> GSNNVLPTWSLDSNGEMRSRLSLSEVLDSGDLMKFAVDKTGCQFLEKAVKGSLTSYQKFQLFEQVIGRKDDFLKLSTNIFGNYLVQSVIGISLATNDDGYTKRQEKLKNFISSQMTDMCLDKFACRVIQSSLQNMDLSLACKLVQALPRDARLIAICVDQNANHVIQKVVAVIPLKNWEFIVDFVATPEHLRQICSDKYGCRVVQTIIEKLTADSMNVDLTSAAQNLRERALQRLMTSVTNRCQELATNEYANYIIQHIVSNDDLAVYRECIIEKCLMRNLLSLSQEKFASHVVEKAFLHAPLELLAEMMDEIFDGYIPHPDTGKDALDIMMFHQFGNYVVQCMLTICCDAVSGRRQTKEGGYDHAISFQDWLKKLHSRVTKERHRLSRFSSGKKMIETLANLRSTHPIYELQSSGHDSFKTDYFSTASEHDGPELEKNGIEEGSLMLEPRSNKSSVSVKFSSSGSHGDD

Caenorhabditis elegans PUF protein fem-3 binding factor-2 (FBF-2) partners with intrinsically disordered Lateral Signaling Target-1 (LST-1) to regulate target mRNAs in germline stem cells. FBF-2 has an architecture characteristic of all PUF proteins, including Drosophila Pumilio and human PUM1 and PUM2. The signature PUF RNA-binding domain (RBD), also called the Pumilio-Homology Domain (PUM-HD), is flanked by extended N-terminal and short C-terminal IDRs. The PUF RBD with eight α-helical repeats recognizes RNA sequence elements.

To explore possible roles of the FBF-2 CT, we expressed and purified an FBF-2 fragment containing both RBD and CT (FBF-2164–632). We determined a crystal structure of FBF-2 RBD + CT in complex with a cFBE RNA (5′-CUGUGAAUG-3′) at 2.1 Å resolution. The electron density map revealed new density, not present in the previous RBD structures. This additional density appeared near a loop in the RBD that connects repeats 7 and 8. The sequence of FBF-2 CT residues 607-613 matched this new electron density, but other C-terminal residues (aa 570-606 and 614-632) were disordered. In the FBF-2 RBD + CT/cFBE crystal structure, the seven visible FBF-2 CT residues (SLMLEPR607–613) align structurally with the core regions of LST-1 A (residues 32-38) and LST-1 B (residues 80-86) and made remarkably similar contacts to the RBD. FBF-2 L610 occupied the same position as the key leucines, L35 and L83, in the LST-1 A and B PIMs, and like LST-1 A L35 and LST-1 B L83, FBF-2 L610 was seated in a hydrophobic binding pocket formed by the Y479, L444, I492, and H482 residues of FBF-2. FBF-2 RBD residues Q448, G478, and I480 contacted the peptide backbone atoms of the FBF-2 CT, LST-1 A, and LST-1 B. Thus, the FBF-2 CT contains an intrinsic PIM. We propose that the FBF-2 PIM acts as Velcro®, attaching to the RBD and constraining the disordered loop to be located near the 5′ end of the bound RNA where an electronegative cluster of acidic residues in the CT weakens RNA-binding affinity by electrostatic repulsion.> MASNDPGNEVSS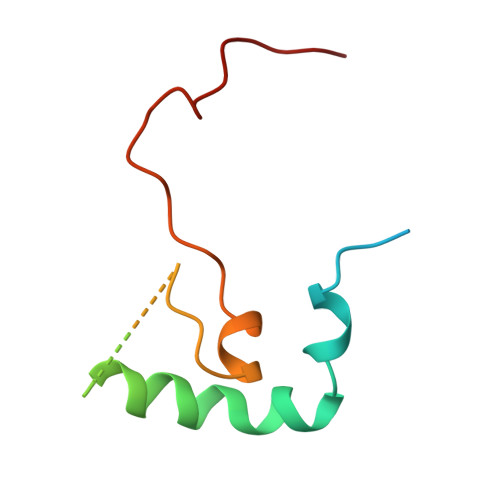YSPTSPSYVKFFTQSNLEKLPKYKEKKAASAKQTAPNNSNGGSEEEITCALDYLIPPPMPKNQQYRAFGSIW2-[(2~{E},6~{E},10~{Z},14~{Z},18~{Z},23~{R})-3,7,11,15,19,23,27-heptamethyloctacosa-2,6,10,14,18-pentaenyl]naphthalene-1,4-dione 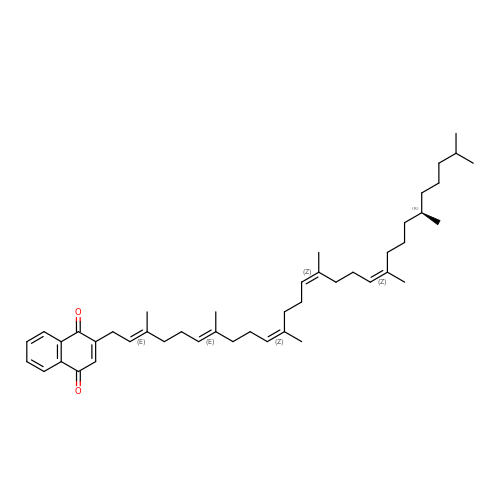| C45 H66 O2 | HQTZEMLTZXAZEE-ZTUUOAHYSA-N>DDKRGRREIRVLHLLEQIRAYCETCWEWQEAHEPGMDQDKNPMPAPVEHQICPAVCVLMKLSFDEEHRHAMNELGGLQAIAELLQVDCEMYGLTNDHYSITLRRYAGMALTNLTFGDVANKATLCSMKGCMRALVAQLKSESEDLQQVIASVLRNLSWRADVNSKKTLREVGSVKALMECALEVKKESTLKSVLSALWNLSAHCTENKADICAVDGALAFLVGTLTYRSQTNTLAIIESGGGILRNVSSLIATNEDHRQI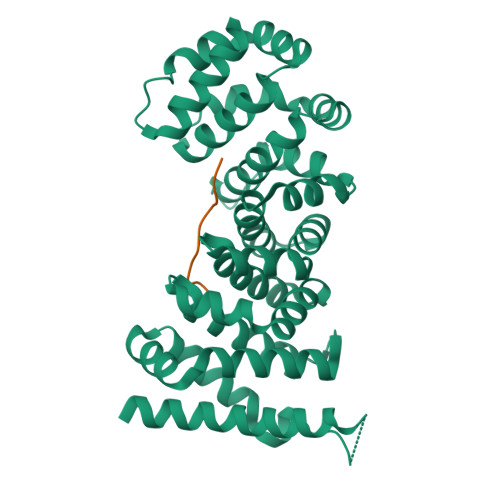LRENNCLQTLLQHLKSHSLTIVSNACGTLWNLSARNPKDQEALWDMGAVSMLKNLIHSKHKMIAMGSAAALRNLMAN[2x];>TYEEYGYDDTYAEQSYEGYEGYYSQSQGDSEYYDYGHGEVQDSYEAYGQDDWNGT[2x]~{N}-[[4-(pyrrolidin-1-ylmethyl)phenyl]methyl]-4-thiophen-2-ylcarbonyl-piperazine-1-carboxamide | C22 H28 N4 O2 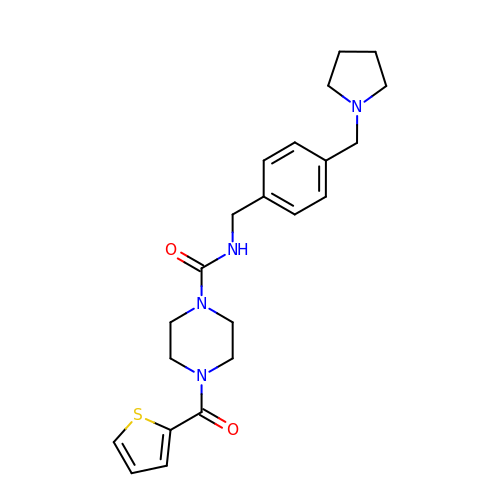S | UTOUOHONUGPBCF-UHFFFAOYSA-N> DHPFTEIKSGFLERRSKFLKSYSKGYYVLTPNFLHEFKTADRKKDLVPVMSLALSECTVTEHSRKNSTSSPNSTGSDAKFVLHAKQNGIIRRGHN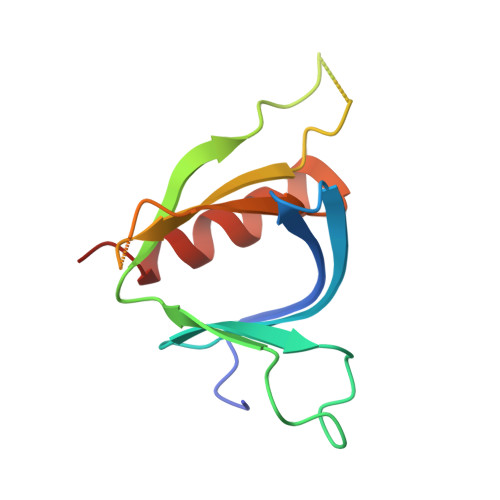WVFKADSYESMMSWFDNLKILTSTS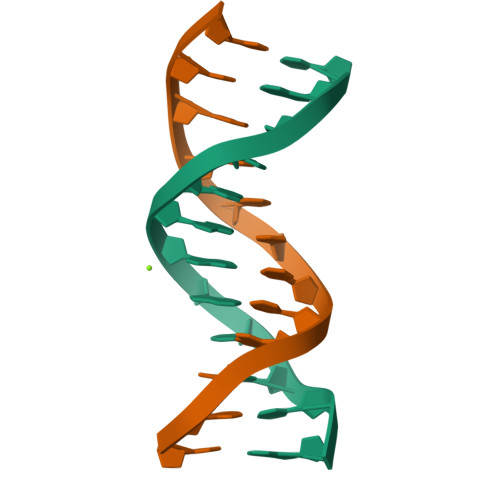>CGCAAAAATGCG[2x];>CGCATTTTTGCG[2x]>SGLVPAGSHMYLSMSISPETINVAGAQRMLSQKMAREALQLRLGAGDPKALAATIAQYERSAADLDAGNAERNVSRMGAPEIAAQRQKVAQIWGRYRAMLDQVAQPASQVDLRGFSQYSTELLGELNNLVSLMSARADSVQHTQMW[3x]

Here we show that Pseudomonas aeruginosa PAO1 mediates nitrate chemotaxis on the basis of specific nitrate sensing by the periplasmic PilJ domain of the PA2788/McpN chemoreceptor. In contrast to the NarX and NarQ sensor kinases, McpN bound nitrate specifically and showed no affinity for other ligands such as nitrite. Following the demonstration that PA2788 specifically binds nitrate, this chemoreceptor was named McpN. No nitrate chemotaxis was observed for the mcpN mutant, suggesting that it is the sole nitrate chemotaxis receptor.

McpN-LBD in complex with nitrate was crystallized in a buffer at pH 7.5, and its structure was resolved by X-ray crystallography to a resolution of 1.3 Å. According to the Matthews coefficient, the unit cell accommodates three chains. Chains A and B of the unit cell form a dimer, whereas chain C forms another dimer with a symmetry-related chain. The McpN-LBD monomer is composed of 4 α-helices that pack into a 4-helix bundle. Dimerization is achieved through the interaction of 22 residues of chains A and B that establish 16 hydrogen bonds and occlude a surface of approximately 1,100 Å2 in each monomer. A single molecule of nitrate is bound to a site with a positive surface charge at the dimer interface. The binding site is situated on the dimer symmetry axis; consequently, the same amino acids from the two monomers establish interactions with bound nitrate. Whereas G58, A59, and M62 establish nonbonded contacts, R61 played a key role in recognition since it forms two hydrogen bonds with nitrate. Taken together, the data indicate that McpN-LBD was present in a monomer-dimer equilibrium and that nitrate binding stabilized the dimeric state. In contrast, a single molecule of nitrate binds to a single site located at the dimer symmetry axis of McpN-LBD.>MQHDLEADVTMTGSDLVSCSYRSLAAPDLTLRDLLDIVETSQAHNARAQLT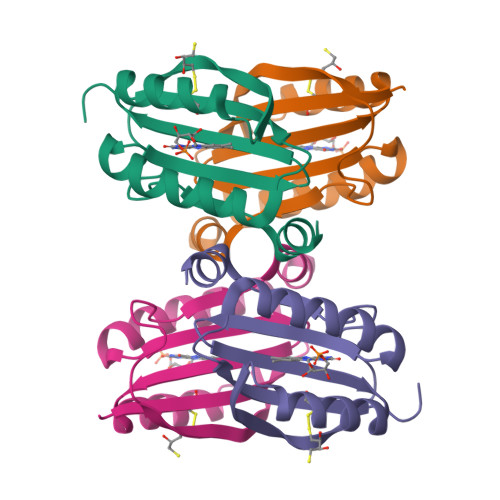GALFYSQGVFFQWLEGRPAAVAEVMTHIQRDRRHSNVEILAEEPIAKRRFAGWHMQLSCSEADMRSLGLAESR[2x]> SSNDNIELVDFQNIMFYGDAEVGDNQQPFTFILDTGSANLWVPSVKCTTAGCLTKHLYD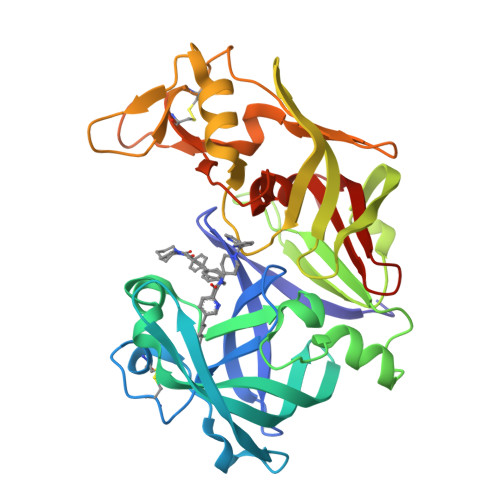SSKSRTYEKDGTKVEMNYVSGTVSGFFSKDLVTVGNLSLPYKFIEVIDTNGFEPTYTASTFDGILGLGWKDLSIGSVDPIVVELKNQNKIENALFTFYLPVHDKHTGFLTIGGIEERFYEGPLTYEKLNHDLYWQITLDAHVGNIMLEKANCIVDSGTSAITVPTDFLNKMLQNLDVIKVPFLPFYVTLCNNSKLPTFEFTSENGKYTLEPEYYLQHIEDVGPGLCMLNIIGLDFPVPTFILGDPFMRKYFTVFDYDNHSVGIALAKKNL> MTTSYEPWPQLYSHLNGTNEEVLDRMKVAELCKGWSVYRDASEWANFKEMFTPDANIWTTWSGAQTIDSFIQISKDGKDKGAFIMHRECGTLVDLNPKTQRAIGKMKTTITQRFEYEGVPFDIDCDNYFIFFCLKDSNGDWKARWYKVFYVKDKFVPVGVPTAENMEKLAKLFSKENLEQYPWGYQYLAVAQANLGYPIDKKLPTWKNEL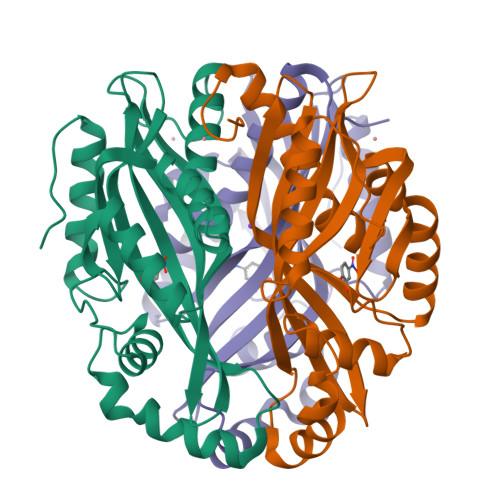YHTMYDAMKEWMEGKEIDLHW> MTNFLNGVNIGTPGAYAFYQTTQSRPINVEPFRTCYMVGFASNGVNKNVPTRISNLTDFTNVYGTSASTNSVDLFFKNSQGFGNLYFVNVAIPTRYQIVVTAATAGSYSVTVNGVTKAITVVGGATTTTIAADVISAINNDTVLNKEVLATVGGTSSTVVITSKKPTNT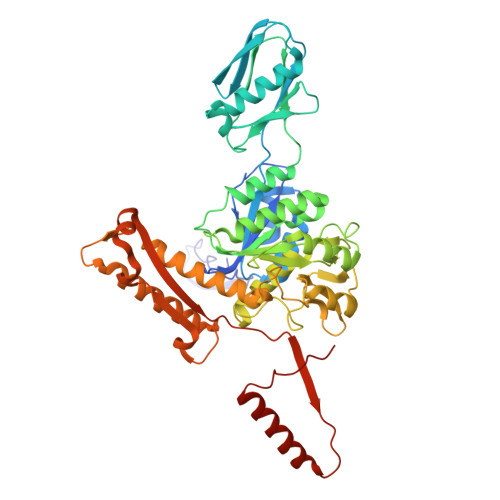TTAAVTGVIFTLTTTTGTSPSVADYVYTINNTFDPALEAGFVIAPEAFSTFTKSDRLSIQVALENLCSAYRYQWAALIDSGAMSEISNTDRAIAEAATYNSVQGHCSYYYPYLINLDDQQVPPSAAVAGMALYRFVIDGFAEPPAGVNFPLKGVKNVAYKVTWEEQNVANPEGVNCILNKENYGIVVWGARTLSADPNIVFISTRIILNIVINTLNRGYDFDIFNSVGGTATVLDNIQRKTNTLLTTLYQAGLFYGQTTSEAFSVLGDASVQVPSLLQQGLVNMFIWVVPSTIIERLIINIKQTAIGDLEATVALDTAALQSSVEEGTATEGTAPVV> MNTAVEPYKASSFDDTHKLTVEKHGHTALITINHPPANTWDRDSLIGLRQLIEHLNRDDDIYALVVTGQGPKFFSAGADLNMFADGDKARAREMARRFGEAFEALRDFRGVSIAAINGYAMGG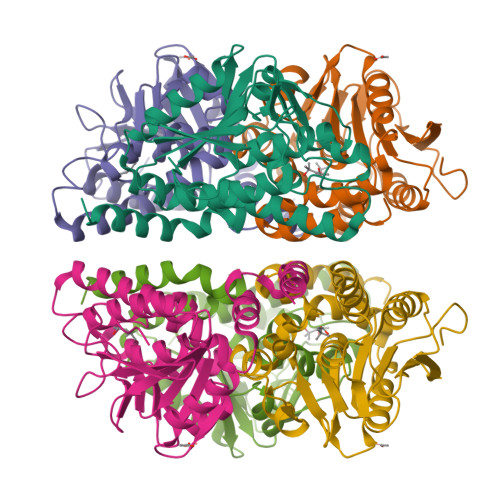GLECALACDIRIAERQAQMALPEAAVGLLPCAGGTQALPWLVGEGWAKRMILCNERVDAETALRIGLVEQVVDSGEARGAALLLAAKVARQSPVAIRTIKPLIQGARERAPNTWLPEERERFVDLFDAQDTREGVNAFLEKRDPKWRNCLEHHHHHH>[6x]MAEYQDKVVDVEVSLGTQPIDTVGFETPMFLAMHGNFPERIRFYVSTAGMVADGFAVGSPAYQFATNAFAGNFAPQRVAIGRMSIDSSKVDFTGTTNTEQVVVNITLNKVVKAVKINVLPGNTPAQIATALADAVTADADLTGKATAVATGTYVTVTAVSPNVVSVGKGAGVYKIVNESSETVATVLPSVIAENHNWYFLATEARSDADIVAAAEFAKANYKLHIYNSTDVDAYAPENSAASVFDTLKSLSYDSLGTSDAGADVDFTEGSVIGAMAANDPSYGDSLHLKTMPGMVPFAGSDTQRSNAWSRNANIYRGLYGGGSYIEGKTSSGQYVDVIRFSHWVKFRMEESVFAYMKRRSDMGLSMKMSDEDLPVLKSVLMNNPINIGIRNGGILTGYDTENKVSYDPTIIIPKRANIPTNDLAARILRDVKVELVYNNSLHYVKIRASVVLDRPAGQSTNAQTPMSSSAVGV;>[4x]NQSKILTLQAYDPAKVLVFIGGQRVSGFAADTKIVITRNNDNISVHAGVDGEISNALSRDNTGVMTLSLQNTAKWNGYLAQWQRQANVTGLIYLPVQVEGSQGLSLNTIGWIQKQPDLSYGTEVGQMDWEIGVLDAWLSPDQIQGIAAGITGLLGL;>MAVNNNSISPAQQAQADKRARDAAAAKRKQDTEVSNAKSREDIQYTMFVSGLRRGRLNEFERKNRTDDLAILFDSVTTHTYTKDYNKSSYAVESKAKASDHVTTQDGKFTFSGTVTDSPYLIDPRNMIDRDTDKENPMLARRPAKAIEILELIADSHQLVTLVTEDNILSNYVITSFQVDRSSEAGSSINVQVTLEEFRFKMVNKTVMARTSDPKKAKNANTGTKQTAEDGAVDDSAKQKRQTPYIGKNAETKERWENAAIGTTDFSGKPGAKLPFDPSDLMRK[2x];>[2x]RTVVRTFDFELSGYPDETFRVVLDSVTYELRFMWNERDESWFMSLGDIGAQRPTITSKLTCYSDILAPYRYLDNVPDGNLYLWPLGDIRTRAGRFNIGPLKGIQMTYSSLIE;>LKDVNHIHPLPDFVRGGFDYVPSDIFSGKENFEQTLRILLERLEFIDQKMVELAELRTTLNAEDAILDEIGRQLGIYRNGLNDPEYRAVIMILTGNNSKSGTRADIIATLKQLFGEDGVTTYKGYNYRLDINIFNTCMEVTDILPEIIDMLPLVTHLRVVENQGY[2x];>MAENYGLTGSGFNLPPMDDLVQETKKTFKSAFGEDFNTESNSVADKLIQIFNEREYQLWLLMGS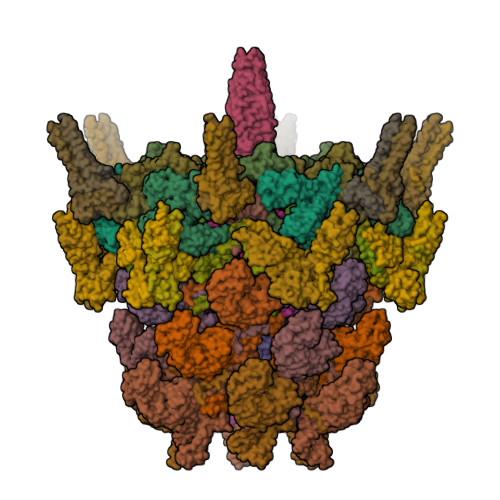VYYAQTMQGAEGIYLDDLLGKRGIYRLGKTRSTGTVVMTIDSSVPYNMIYSAATYTIDTDYELSSDVQVAGNIVAQLIKGTDLSVGTYRLQIQNTTDQSVKTLSLNLTATSGQPLITFFGQIKDFIVNNTILSNQDRIWIDSTEGALYIGYDTNKIMIGLSSRVDFRTNPMAGTRSISMDVRSIEPGYISRDVHSVRSINPTPGGFVDIDNLSAFIDGSDVESDNEYRIRAATSISEGKATRPAILAALLNKVEGIEKVRIFNNNTDKTNSLGIPPYRFMVVCYGGGTAEISQVLYDTIATSNNTYGDTFYDITTEDDQVERIWHTKAAARQLAIRVRYRGRPLSLTEETAIANGLATAVNGTMIAGTLYNVRLVGTVMSSTSPDRFTQVYVDIKNKGQPDSAYVNTDVTASTTQVLSLELEDVIFSQIV[4x];> MAASGNVVVTRTTNRVTFETDKASYARAVKQIRQVGKEWEKASDAISKPKKDPAKAYDKSAQQMRLVNKRLAETRAREEKRASERSIALARREAKAKEAIARVSAARIKQQVQQMTSPRAGMSEMKKFYQQQEREAKKANRKATIGMNAASRPMNVTRINSAPLSPRGGQGTGMVGDPNKVYNPELIAAQNRAMAGRIRSQSQAQDRKAKAEARQRAAAAARAARIDDVMAQQRIRLSSKYGRSYEGRLGRDGAGQGIQDLNRQFRAGTLSAGQYRQSIQALERQFRSAQANAGGFGAALGDIRSQLLNAGAAYGVFASGASVLKQGQFFQGMEATMSMVSDSSEEAGQRIKFVKDQAYRLGLDLKIASQGYTQMAVNSAGILSKAQNDDLFKGFSEFATASQVDPVKFQRGITAIGQMMGKGQVMAEELKGQLAEGIPGSLQVFVKAAQEAFGDTTIDVEKLMDMMQKGELKAAKILPFVGKYFAEAARKGGALPKALESNRVAMQRLSLTWIDFQNQIFQGGFGEQMTRVFRDLATILDSNGELATNLGAFFGNVIEGFWDMVTEIHDDFVLLDRIVSYYTEKLGYQGDLLKEVFDWAGYAIGIGIFVGGLNKIFKILTKIAGLRTALVGVRQAMGGAITRGGVTNGAGLGGGAGAAGTPGASRTASFLSKWKGLSKISKVGILGTLYSAGSMLNEQFIKRGDDKLADAGLDQETFQKEYGFMPKPVGLLDVFDKWFNKPRDLDAPTITAPGPGSGMAAQTGIPFPAPQKVEGDITIKIEAGELRNMVRAVVDENNQFNFNMLIQGGPN;> MRAMERTYTLVIGRPVVIGEKPVNIEKFANTSKGDAYEIKDLHIEFNVKKDNSKEPNKGYVTVYNLSDEVVNYLSVNQRESLAVMLHAGYNGDEKLIFSGTVEYVEDDFPEETRTTKFILGDGTLNLTTATTARSYRKGTPVNSVLNDLIADLKLPKGRVIDFGNQTLQTSMAFTGNASQNLANLAKNTGSTFSVQDGAVYWTKEGSRFNNVMFEISEEGGMVGTPTPKQPSSSKKLIKAKAKAKSDEAEGKKPKAPSKKKKEHDIKEDVGMTVSTLLNGAILPESTVYLNTRYHKGFYKVAELTHRGGYETGDWITELGLVETRGELIK;> MAYADRYDAAFGIYISRFLRNNVHTNIRGKVVGVNYSGPSVDVQPMAYTEFPSGTTDRYPVIYDVPVLLPSGAGGKARLTMPIKPGDVVGLSFSERNEGDNNDQNTHQLFAGWAVTQIFTDGNSKAIHPDNVVLENDKAIITLKPDGDTSLQNPKVTVEALADGNVKISNGTGEFTMSPSGEIKGGNRGGSFTLQPSGQLMCNGARITTSGRIITANGVDMDDFYQKYMSHTHGGVSRGGDNTNPPN;>MAKPKDPIYVWAAADVNLPGTGRPNKSKPIDDLLAKGYDKGQKPAAEEFNYILNMSSAWVNWIVNEKFPELEAEIARLLAELENRINQQLAVIRQDIAQLRQDVADLRRYVDQKVQELKQEIQGVRNDLNKLRQDFDAAITQVNGRIDDLEPRLVPIGAVIPWPGATVPDGWLECSGQVFNTGQNPKLYSVLGRNVVPDYRGLFLRGWAHGSDANDPDAGRALGSVQGDAIRNITGYFPADIGNSNFIGRYVGGAFRDDGSLTSGDDGTRSNEVRKYSFDASREVPVAAENRPKNIAVMYIIKTDQAQSSGGNSPTAIVVSPDTITNRIGYAVKATASVLPASISGQYPISWSTQNAAVATVDGSGNISLVGPGETNIIASISTGMNVVIRVTSYSVLTSISIADPGQITVTESKMLVVTKSPSSANEPLQFLSNNSGVAAVNDAGYVIGVSAGSATITVRGTLSGVSSTRAVTIIPEQVEESVQDNRLGAVGSYIPPSPSSNVMSWTFQAPQGCALTGIIVQENESNSGDNIGGVYYKPIQKKVNGVWVTITG[6x];>[6x]MSSNTDIIALLSSDADKAVDQIIEDSKRLHIVVNGTGTEQAVAEDGSLLPSVRKALIDNLYFKTPPLPWRNGGSVNEFNQLYSFTDVSGNTTWWYAPGATVSNPVVMRDSPINDGKFKVFLDKTNIADIYAPLNSPNFVGNPRVPTPAPGDNSQSIPTTGWVQSEMEGLEDLIISSMRGEFENITVRNDAILQDTYINGEFIVTSDKLAAANTEATFRRIRMVGTGTTGTAATEIAFEQNTTPPPGVSTKTNIKPFAVSTGILTVDQINGKAAQVGDVAVSTDSLNVDGYMRGDYLHLEGNNRNTAGRPQLIVDGIAEIETLRVTGTIEGVKADVDGLDIHPRSVIVDEGLTVAKDTTMTGKLTVGGTTKVGNLEVTGTLSGVAISVDGKDIKPRSVNTGNLVATGDVQISGTTTATGKITTQDLEVLGTLTANLDLSGSDLSVDNINVAQTATITDLVVTGTTTGVKGDVEGEAIAPASVAATGTVSAASMSTTGNMAVGGNLTITGDFRPASVAGQDTPRLVVQGDSDLQGDLNVSGTITGVVDLTAQDINMNSLGLAQGLTAGGGITSFSTVKGVNGVFGEGSTAPGAIGLQSMTNAKVATDLLVGEDLRVEGDTNLFGNLSVTGTITGNMNFSGKTIAPATVNATTVTATNLTVTGTIDLTDSPIVAQEITATNVEATGKMVAGKYSTTPKTANATTATFTPDGTTSIYNVNVQADTEVQAPAGLLSSGKGESIFIYFEQDTTGHAVTFSSAFVVHNAATVSNAANSITIANLVYRGTGPLIDVFLTGR;>[2x]QFKDLLLDPLTGDLDFGTPGDRGMRLALTNQLSLRQRLYLRFAIWAGDWYFDETFGFPYRTFVGKKTVKAVLDGRIKSEVRQEPDVLQITDFQSTMDVVSRSYKCFFTVVTAEGEEISLAFVGEDEYQYPTPPESNVQLCGDEGVIINFKNKLYYLINFRLPK> GSHGMTEAASEGTESFAFGAVVERRDELDGRPWISYPVRVVADTPELVAVHLSHGTRLTFGDDPFSWGPHPWQLFGDRWQSAGILQLHRPGRGHSVWVLRDADTGAFREWYVNVEAPWRRTPTGFSTLDHEIDLVVPADSRTFRWKDVEKFEERARIGHFSPEEATAIRAEAADVAREIAAGEQ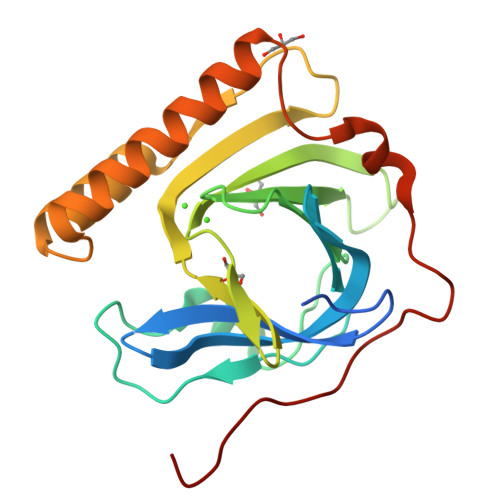WWDTRWSRWEPPAGWNALLQSFETEGS> IRNTNEYTEGP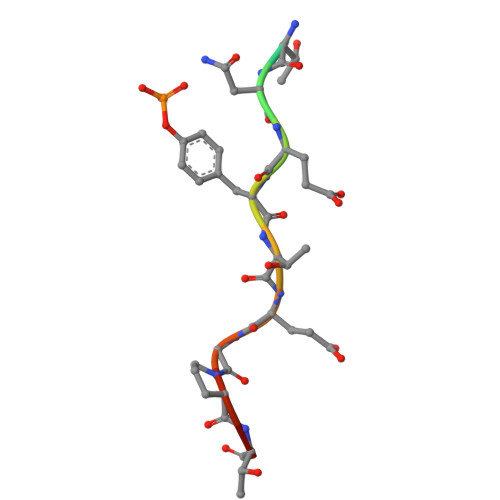TV>[2x]ASQPNSSAKKKEEKGKNIQVVVRCRPFNLAERKASAHSIVECDPVRKEVSVRTGGLADKSSRKTYTFDMVFGASTKQIDVYRSV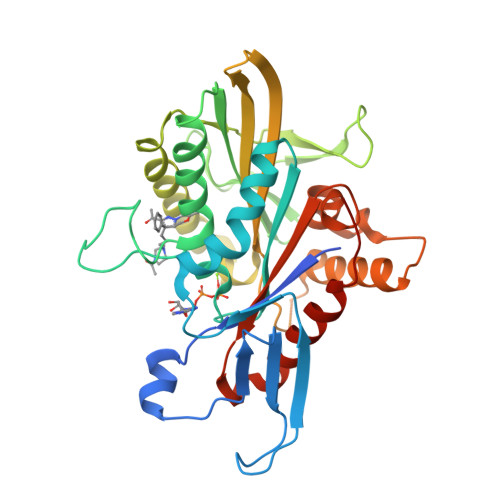VCPILDEVIMGYNCTIFAYGQTGTGKTFTMEGERSPNEEYTWEEDPLAGIIPRTLHQIFEKLTDNGTEFSVKVSLLEIYNEELFDLLNPSSDVSERLQMFDDPRNKRGVIIKGLEEITVHNKDEVYQILEKGAAKRTTAATLMNAYSSRSHSVFSVTIHMKETTIDGEELVKIGKLNLVDLAGSENIGRSGAVDKRAREAGNINQSLLTLGRVITALVERTPHVPYRESKLTRILQDSLGGRTRTSIIATISPASLNLEETLSTLEYAHRAKNILNKPEVNQK> VGVNPLPAPREISWGSSGPKSIAGELQLRTDSDSADGIVADAWNRAWETIVAL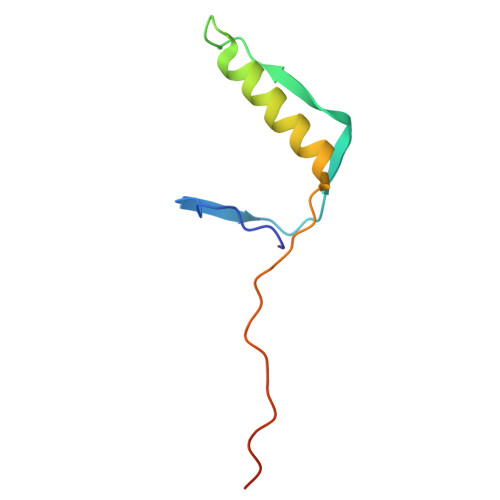RWVPAATEAPISSFEPFPTPTAGAS> 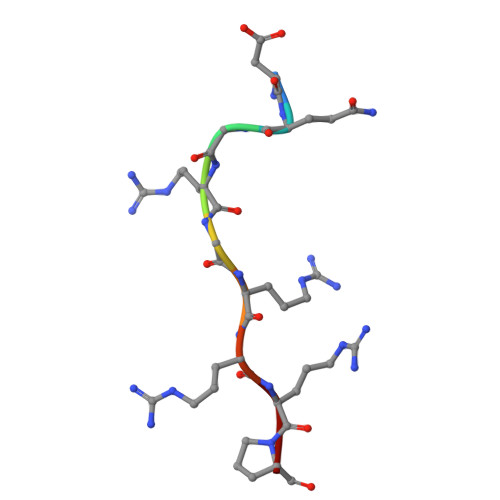DQGRGRRRP> MAEARSQPSAGPQLNALPDHSPLLQPGLAALRRRAREAGVPLAPLPLTDSFLLRFLRARDFDLDLAWRLLKNYYKWRAECPEISADLHPRSIIGLLKAGYHGVLRSRDPTGSKVLIYRIAHWDPKVFTAYDVFRVSLITSELIVQEVETQRNGI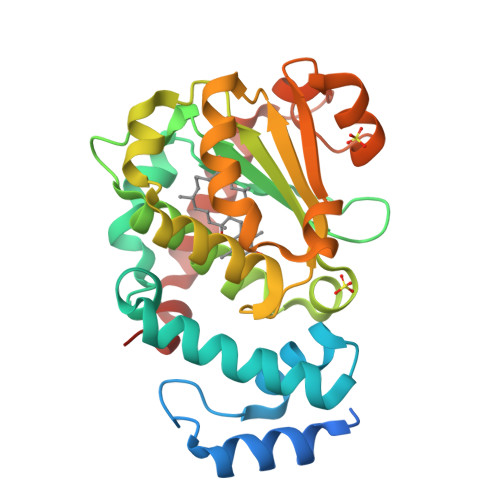KAIFDLEGWQFSHAFQITPSVAKKIAAVLTDSFPLKVRGIHLINEPVIFHAVFSMIKPFLTEKIKERIHMHGNNYKQSLLQHFPDILPLEYGGEEFSMEDICQEWTNFIMKSEDYLSSISESIQ> MSADNGLIIGIDLGTTNSCVSVMEGGRPVVLENPEGKRTTPSIVSYKNNEIIVGDAAKRQMVTNPNTIVSIKRLMGTSNKVKVQNADGTTKELSPEQVSAQILSYLKDFAEKKIGKKISRAVITVPAYFNDAERNATKTAGKIAGLNVERIINEPTAAALAYGIDKASREMKVLVYDLGGGTFDVSLLDIAEGTFEVLATAGDNRLGGDDWDNKIIEYISAYIAKEH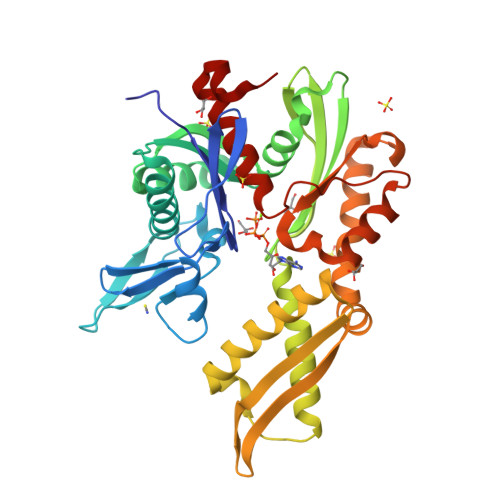QGLNLSKDKMAMQRLKEAAERAKIELSAQLETIISLPFLTVTQKGPVNVELKLTRAKFEELTKPLLERTRNPISDVIKEAKIKPEEINEILLVGGSTRMPAVQKLVESMVPGKKPNRSINPDEVVAIGAAIQGGVLRGDLEHHHHHH2-amino-2-deoxy-1-O-phosphono-alpha-D-glucopyranose 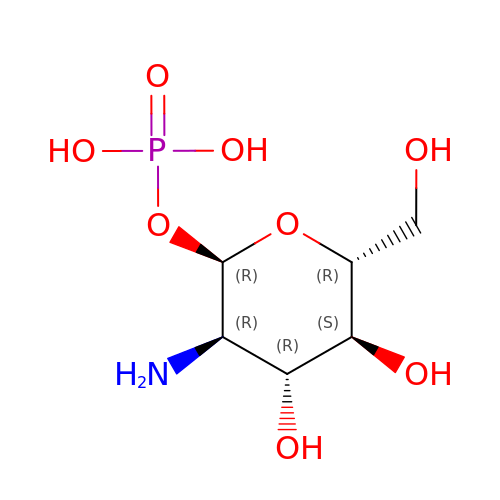| C6 H14 N O8 P | YMJBYRVFGYXULK-QZABAPFNSA-N>[4x]MTHHYPTDDIKIKEVKELLPPIAHLYELPISKEASGLVHRTRQEISDLVHGRDKRLLVIIGPCSIHDPKAALEYAERLLKLRKQYENELLIVMRVYFEKPRTTVGWKGLINDPHLDGTFDINFGLRQARSLLLSLNNMGMPASTEFLDMITPQYYADLISWGAIG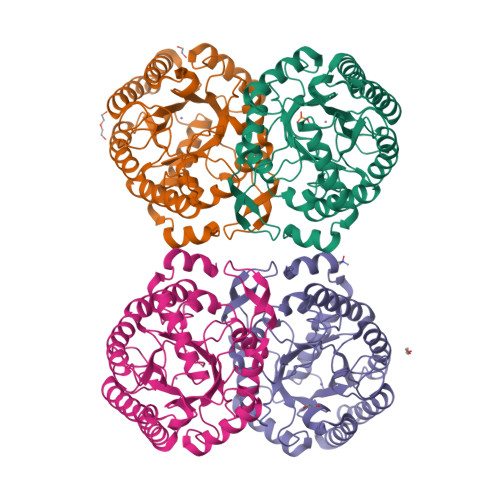ARTTESQVHRELASGLSCPVGFKNGTDGNLKIAIDAIGAASHSHHALSVTKAGHSAIVHTGGNPDCHVILRGGKEPNYDAEHVSEAAEQLRAAGVTDKLMIDCSHANSRKDYTRQMEVAQDIAAQLEQDGGNIMGVMVESHLVEGRQDKPEVYGKSITDACIGWGATEELLALLAGANKKRMARAS> EAAHGISGGTIIYQLLMFIILLALLRKFAWQPLMNIMKQREEHIANEIDQAEKRRQEAEKLLEEQRELMKQSRQEAQALIENARKLAEEQKEQIVASARAEAERVKETAKKEIEREKEQAMAALREQVASLSVLIASKVIEKELTE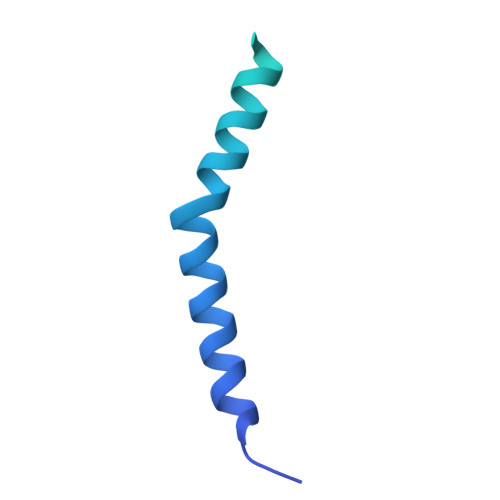QDQRKLIEAYIKDVQEVGGAR>[8x]THPDISVDVLVIGAGPTGLGAAKRLNQIDGPSWMIVDSNETPGGLASTDVTPEGFLYDVGGHVIFSHYKYFDDCLDEALPKEDDWYTHQRISYVRCQGQWVPYPFQN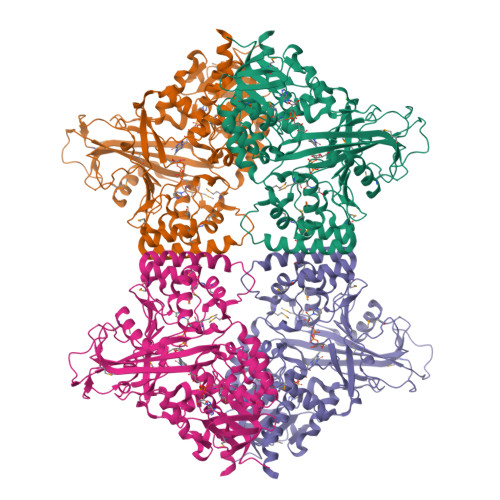NISMLPKEEQVKCIDGMIDAALEARVANTKPKTFDEWIVRMMGTGIADLFMRPYNFKVWAVPTTKMQCAWLGERVAAPNLKAVTTNVILGKTAGNWGPNATFRFPARGGTGGIWIAVANTLPKEKTRFGEKGKVTKVNANNKTVTLQDGTTIGYKKLVSTMAVDFLAEAMNDQELVGLTKQLFYSSTHVIGVGVRGSRPERIGDKCWLYFPEDNCPFYRATIFSNYSPYNQPEASKKLPTMQLADGSRPQSTEAKEGPYWSIMLEVSESSMKPVNQETILADCIQGLVNTEMLKPTDEIVSTYHRRFDHGYPTPTLEREGALTQILPKLQDKDIWSRGRFGSWRYEVGNQDHSFMLGVEAVDNIVNGAVELTLNYPDFVNGRQNTERRLVDGAQVFAKSKAQ>[4x]GSHMTDPSKLAVAVVDSSNMNRSMEAHNFLAKKGFNVRSYGTGERVKLPGMA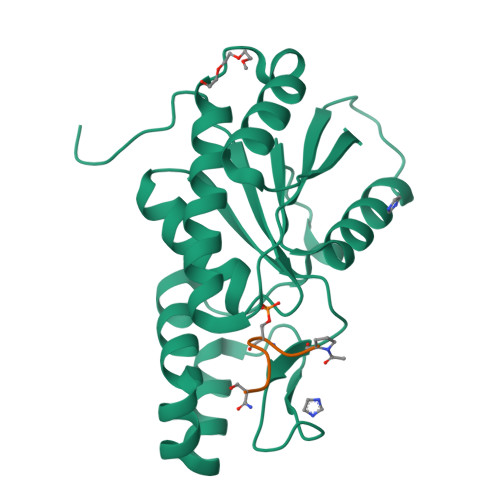FDKPNVYEFGTKYEDIYRDLESKDKEFYTQNGLLHMLDRNRRIKKCPERFQDTKEQFDIIVTVEERVYDLVVMHMESMESVDNRPVHVLNVDVVNNAEDALMGAFVITDMINMMAKSTDLDNDIDELIQEFEERRKRVILHSVLFY;>PTSPSYS[4x]> MKTFIFLALLGAAVAFPVDDDDKIVGGYTCGANTVPYQVSLNSGYHFCGGSLINSQWVVSAAHCYKSGIQVRLGEDNINVVEGNEQFISASKSIVHPSYNSNTLNNDIMLIKLKSAASLNSRVASISLPTSCASAGTQCLISGWGNTKSSGTSYPDVLKCLKAPILSDSSCKSAYPGQITSNMFCAGYLEGGKDSCQGDSGGPVVCSGKLQGIVSWGSGCA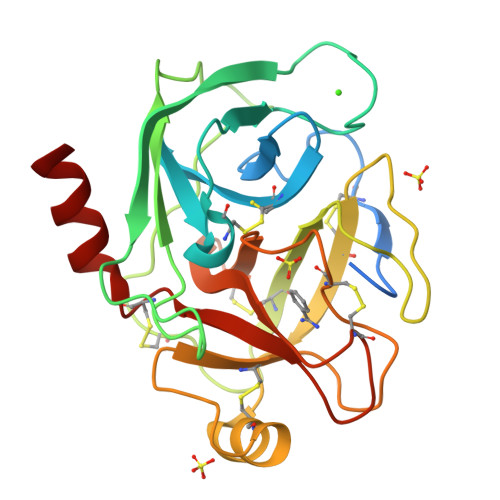QKNKPGVYTKVCNYVSWIKQTIASN> MGSSHHHHHHMPFTIDSARGIFPNTLAADVVPATIARFSQLNAEDQLALIWFAYLEMGKTLTIAAPGAASMQLAENALKEIQAMGPLQQTQAMCDLANRADTPLCRTYASWSPNIKLGFWYRLGELMEQGFVAPIPAGYQLSANANAVLATIQGLESGQQITVL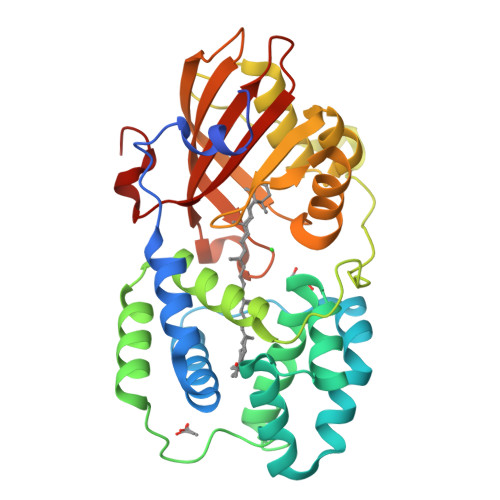RNAVVDMGFTAGKDGKRIAEPVVPPQDTASRTKVSIEGVTNATVLNYMDNLNANDFDTLIELFTSDGALQPPFQRPIVGKENVLRFFREECQNLKLIPERGVTEPAEDGFTQIKVTGKVQTPWFGGNVGMNIAWRFLLNPEGKIFFVAIDLLASPKELLNFAR> NMLYHRYLKPNSEYYKKIEVRGKDNIYELNDIPDTYAVFLDNESVWKHYHVKGSTLPEQGWKIHVTSSLEDSKDVLDKVARLCIDKKIEFKHLKDKDSFMKMNSKNANRASSGKFITIYPTNNEVFVELLEMISLAIQDFKKGPYILNDKRWKNSNVFYRYGGFKGIFNEHGEHCIRDKEGNLIKDQRNPFYQVPDFVKDFDDYLNTINNSGELENKGESRLGKYKIETALSFSNAGGVYLATRKKDNLKVIIKEARPSAGLDGAAQDALARQKIEYDALKKLK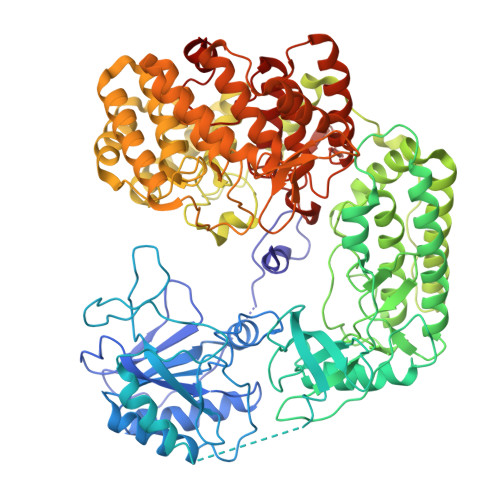DVSGVVNLIEYFQEWEHYFLVEEFIEGRDLRQWIAQEFPFFEDNNGMSNHIKDVKMILLQLLDLIDSMHNQGVAMGDLQPANIMVTEDLTVRIIDFETAMPVNSDDRPAMLTTGFVSHEMKVSGARDWFGFKRLVRYLALPVLTSEDLEGYLQYNHLNWIKENYGYEFYSFIVDLQEKCDKRIKDYQTFIPKEINLNDQTSDFNLTSIINKLIIGVESSLTNDERFINGDIRQFEMNGGKFNFLTGGSGAAFTLTKNKSSIAEVDKWIQSVLLDNLPLIEEDGLFTGKTGILALLYDKGYKEVVLNELKILKDNINQTDISIRSGLSGIGLFVISLYLETENKEYLKLAKDLERMIKLNRAKDKQLKVKDWMAVDIGVIDGLSGVSLFYSALYSVTQNQKYLEEAEVLIKEDLESTKKDDVTGVLQTVDNKNRLLPYLSGGSIGVAISIWFLNHVSGQDLYREEMNSILKLSKTRCTISGGLFDGAGSFLLIPSMVKNDKNREVILNEVLNLLNIFLIEKNSYYVYPGQFSYRLADDVYTGSSGIILALMGVIKGNPLYWLPLVNSDEFLARTKV> SKTKPFSLPILTISELTNSRFPAPIDSLYTAQNNNLNVQCQNGRCTLDGELQGTTQLLPSGICAFRGKLTADVHQSHDDRWHMQLTNLNGTPFDPTEDVPAPLGTPDFTGLLFGVASQRNVVSNPNTTRAHEAVISTTSSQFVPKLGSINFGSTSDDFQLQQPTKFTPVGIKVESGHDFDQWAPPRYSGHLTLNMNLAPPVAPN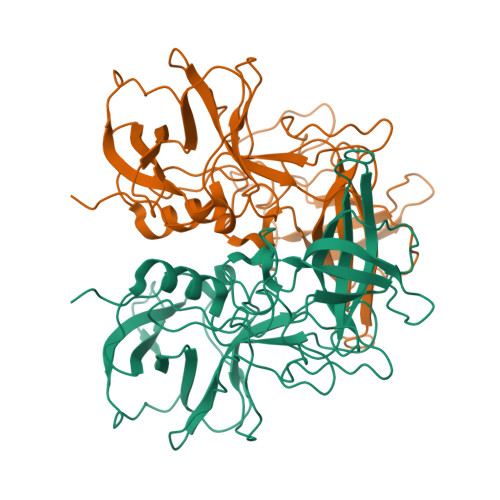FPGEQLLFFRSNVPCAGGVSDGVIDCLLPQEWIQHFYQESAPSQSDVALIRYVNPDTGRTLFEAKLHRTGYITVAHSGDYPLVVPSNGYFRFDSWVNQFYSLAPM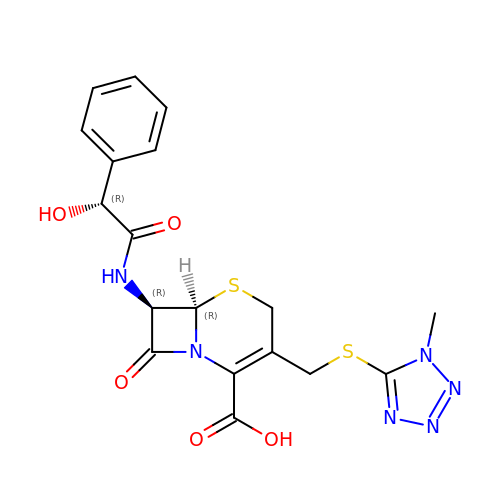(6R,7R)-7-{[(2R)-2-hydroxy-2-phenylacetyl]amino}-3-{[(1-methyl-1H-tetrazol-5-yl)sulfanyl]methyl}-8-oxo-5-thia-1-azabicyclo[4.2.0]oct-2-ene-2-carboxylic acid | C18 H18 N6 O5 S2 | OLVCFLKTBJRLHI-AXAPSJFSSA-N>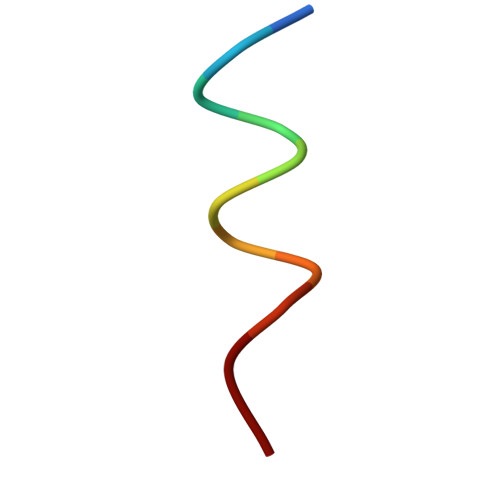 GAFQNLFQSVR1-(3-methoxyphenyl)-1,2,3,4-tetrazole | C8 H8 N4 O | 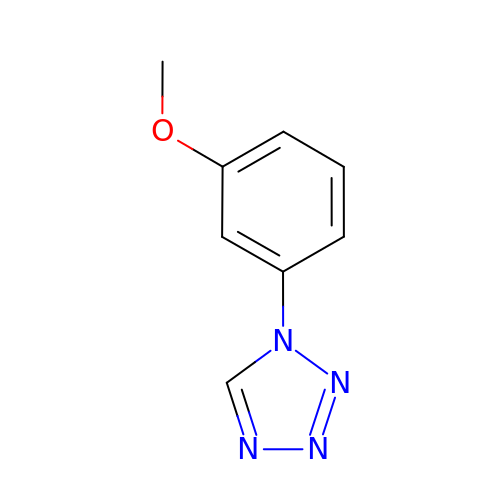MDTADZVGCMQTQW-UHFFFAOYSA-N>[2x]HHHHHHMAEVKLYGFWPSPFSHRIIWALKLKGVEYEYIEEDLSNKSESLLKYNPVYKKIPVLVHGDKPIAE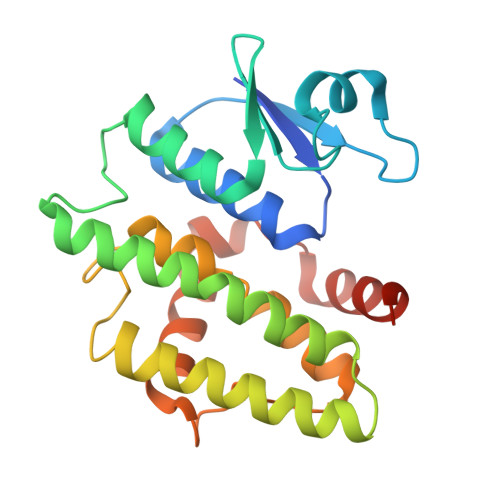SLVILEYIEETWPENPLLPKDPYERAMARFWIQYGVDTVAALRAFYLGSGEELEKAAKELSECLKILEEQGLGDKKFFGGESMNLVDISYGALGYWLAAVEEAKGVTVLKPSTLPRLHAWAKNLDELPVVKENIPASDKMLAYVTAAMNRPAKN> MTARGLALGLLLLLLCPAQVFSQSCVWYGECGIAYGDKRYNCEYSGPPKPLPKDGYDLVQELCPGFFFGNVSLCCDVRQLQTLKDNLQLPLQFLSRCPSCFYNLLNLFCELTCSPRQSQFLNVTATEDYVDPVTNQTKTNVKELQYYVGQSFANAMYNACRDVEAPSSNDKALGLLCGKDADACNATNWIEYMFNKDNGQAPFTITPVFSDFPVHGMEPMNNATKGCDESVDEVTAPCSCQDCSIVCGPKPQPPPPPAPWTILGLDAMYVIMWITYMAFLLVFFGAFFAVWCYRKRYFVSEYTPIDSNIAFSVNASDKGEASCCDPVSAAFEGCLRRLFTRWGSFCVRNPGCVIFFSLVFITACSSGLVFVRVTTNPVDLWSAPSSQARLEKEYFDQHFGPFFRTE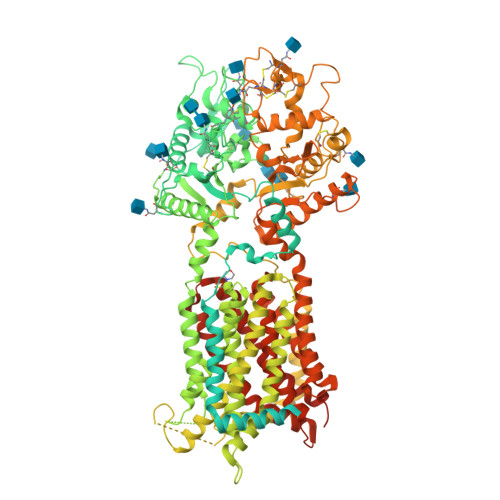QLIIRAPLTDKHIYQPYPSGADVPFGPPLDIQILHQVLDLQIAIENITASYDNETVTLQDICLAPLSPYNTNCTILSVLNYFQNSHSVLDHKKGDDFFVYADYHTHFLYCVRAPASLNDTSLLHDPCLGTFGGPVFPWLVLGGYDDQNYNNATALVITFPVNNYYNDTEKLQRAQAWEKEFINFVKNYKNPNLTISFTAERSIEDELNRESDSDVFTVVISYAIMFLYISLALGHIKSCRRLLVDSKVSLGIAGILIVLSSVACSLGVFSYIGLPLTLIVIEVIPFLVLAVGVDNIFILVQAYQRDERLQGETLDQQLGRVLGEVAPSMFLSSFSETVAFFLGALSVMPAVHTFSLFAGLAVFIDFLLQITCFVSLLGLDIKRQEKNRLDIFCCVRGAEDGTSVQASESCLFRFFKNSYSPLLLKDWMRPIVIAIFVGVLSFSIAVLNKVDIGLDQSLSMPDDSYMVDYFKSISQYLHAGPPVYFVLEEGHDYTSSKGQNMVCGGMGCNNDSLVQQIFNAAQLDNYTRIGFAPSSWIDDYFDWVKPQSSCCRVDNITDQFCNASVVDPACVRCRPLTPEGKQRPQGGDFMRFLPMFLSDNPNPKCGKGGHAAYSSAVNILLGHGTRVGATYFMTYHTVLQTSADFIDALKKARLIASNVTETMGINGSAYRVFPYSVFYVFYEQYLTIIDDTIFNLGVSLGAIFLVTMVLLGCELWSAVIMCATIAMVLVNMFGVMWLWGISLNAVSLVNLVMSCGISVEFCSHITRAFTVSMKGSRVERAEEALAHMGSSVFSGITLTKFGGIVVLAFAKSQIFQIFYFRMYLAMVLLGATHGLIFLPVLLSYIGPSVNKAKSCATEERYKGTERERLLNF> ANTSSAYNSVYDFLRYHDRGDGLTVNGKTSYSIDQAAAQITRENVSWNGTNVFGKSANLTFKFLQSVSSIPSGDTGFVKFNAEQIEQAKLSLQSWSDVANLTFTEVTGNKSANITFGNYTRDASGNLDYGTQAYAYYPGNYQGAGSSWYNYNQSNIRNPGSEEYGRQTFTHAIGHALGLAHPGEYNAGEGDPSYNDAVYAEDS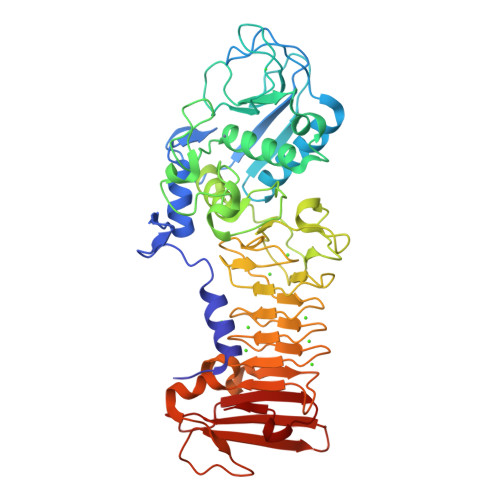YQFSIISYWGENETGADYNGHYGGAPMIDDIAAIQRLYGANMTTRTGDSVYGFNSNTDRDFYTATDSSKALIFSVWDAGGTDTFDFSGYSNNQRINLNEGSFSDVGGLKGNVSIAHGVTIENAIGGSGNDILVGNSADNILQGGAGNDVLYGGAGADTLYGGAGRDTFVYGSGQDSTVAAYDWIADFQKGIDKIDLSAFRNEGQLSFVQDQFTGKGQEVMLQWDAANSITNLWLHEAGHSSVDFLVRIVGQAAQSDIIV>MALSTATKAATDALAANRAPTSVNAQEVHRWLQSFNWDFKNNRTKYATKYKMANETKEQFKLIAKEYARMEAVKDERQFGSLQDALTRLNAGVRVHPKWNETMKVVSNFLEVGEYNAIAATGMLWDSAQAAEQKNGYLAQVLDEIRHTHQCAYVNYYFAKNGQDPAGHNDARRTRTIGPLWKGMKRVFSDGFISGDAVECSLNLQLVGEACFTNPLIVAVTEWAAANGDEITPTVFLSIETDELRHMANGYQTVVSIANDPASAKYLNTDLNNAFWTQQKYFTPVLGMLFEYGSKFKVEPWVKTWDRWVYEDWGGIWIGRLGKYGVESPRSLKDAKQDAYWAHHDLYLLA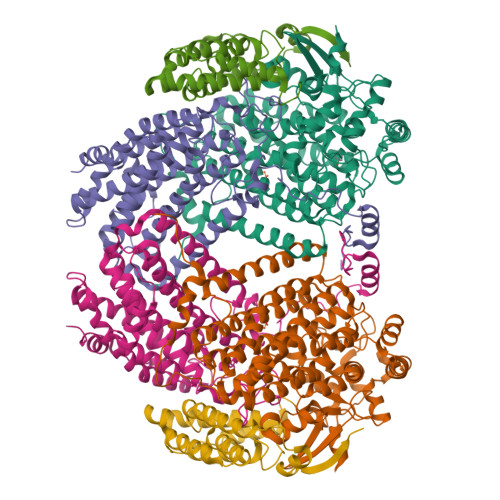YALWPTGFFRLALPDQEEMEWFEANYPGWYDHYGKIYEEWRARGCEDPSSGFIPLMWFIENNHPIYIDRVSQVPFCPSLAKGASTLRVHEYNGEMHTFSDQWGERMWLAEPERYECQNIFEQYEGRELSEVIAELHGLRSDGKTLIAQPHVRGDKLWTLDDIKRLNCVFKNPVKAFN[2x];>[2x]MSMLGERRRGLTDPEMAAVILKALPEAPLDGNNKMGYFVTPRWKRLTEYEALTVYAQPNADWIAGGLDWGDWTQKFHGGRPSWGNETTELRTVDWFKHRDPLRRWHAPYVKDKAEEWRYTDRFLQGYSADGQIRAMNPTWRDEFINRYWGAFLFNEYGLFNAHSQGAREALSDVTRVSLAFWGFDKIDIAQMIQLERGFLAKIVPGFDESTAVPKAEWTNGEVYKSARLAVEGLWQEVFDWNESAFSVHAVYDALFGQFVRREFFQRLAPRFGDNLTPFFINQAQTYFQIAKQGVQDLYYNCLGDDPEFSDYNRTVMRNWTGKWLEPTIAALRDFMGLFAKLPAGTTDKEEITASLYRVVDDWIEDYASRIDFKADRDQIVKAVLAGLK;>[2x]MAKLGIHSNDTRDAWVNKIAQLNTLEKAAEMLKQFRMDHTTPFRNSYELDNDYLWIEAKLEEKVAVLKARAFNEVDFRHKTAFGEDAKSVLDGTVAKMNAAKDKWEAEKIHIGFRQAYKPPIMPVNYFLDGERQLGTRLMELRNLNYYDTPLEELRKQRGVRVVHLQSPH1H-pyrazolo[3,4-d]pyrimidin-4-amine | C5 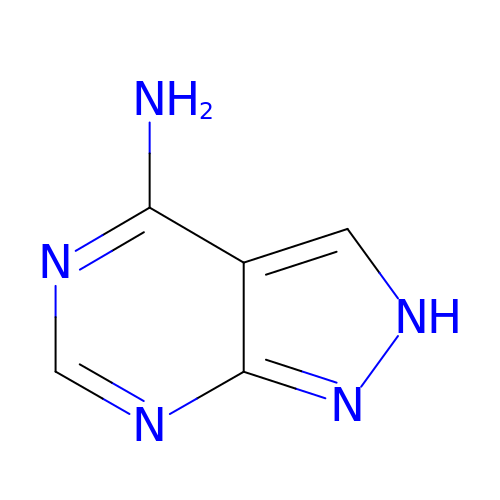H5 N5 | LHCPRYRLDOSKHK-UHFFFAOYSA-N> GAGCAGACTTG;> ACAG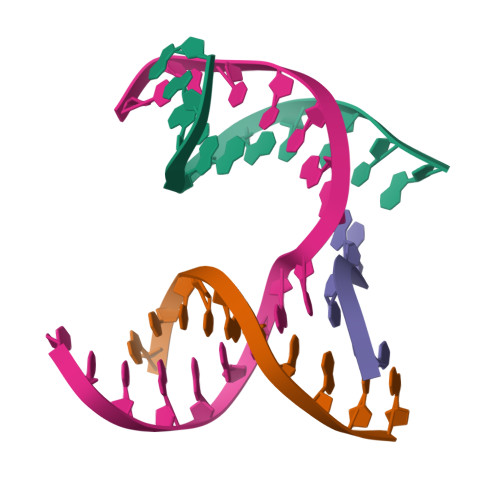CACTCA;> CATGT;> TCTGAGTGCAGTCTGC Enolase, a ubiquitous enzyme, catalyzes the reversible conversion of 2-phospho­glycerate (2PG) to phospho­enolpyruvate (PEP) in the glycolytic pathway of organisms of all three domains of life. Here we present structural snapshots of Mycobacterium tuberculosis (Mtb) enolase in apo, PEP-bound and two 2PG-bound forms as it catalyzes the conversion of PEP to 2PG. MtEno has a topology similar to other enolase structures, a smaller N-terminal domain and a larger C-terminal domain. The crystal and the cryoEM structures (enzyme in solution, frozen) along with the biochemical studies clearly demonstrate that the functional unit of MtEno is an octamer.

Tautomerization resonance is accelerated on acidification of the carboxyl group of 2PG which is accomplished through its lone-pair-mediated coordination with both the Mg2+ ions and the transfer of a proton from His154 onto the nearest oxygen linked to the phosphate moiety. To find out if the exact reverse of this reaction occurs during the conversion of PEP to 2PG, we systematically mutated each of the residues Ser42, Asp241, Glu163, Glu204 and Lys335 to alanine, compared their activity with wild type MtEno, and elucidated the structures of three of them [Figs. 4(a) and 4(b)]. Notably, the K335A mutation disrupts the nucleophilic (proton) substitution, the E204A mutation defuncts enolation capacity, D241A should make the MgA 2+ coordination in the active site highly improbable and S42A should absolve the MgB 2+ coordination. We analyzed the solvent accessibility in the protein structure based on tunnels and channels buried in the core of the protein by employing CAVER. The water-accessibility channel tunnel of the MtEno S42A–2PG co-crystal structure was similar to that of MtEno Wt-2PG [Figs. 4(d) and 4(e)], corroborating our annotation of the substrate being 2PG. On the other hand, MgB 2+ was absent, possibly owing to the role of Ser42 in MgB 2+ coordination. However, conversion of PEP to 2PG even in its absence indicated that MgB 2+ may be non-obligatory for the reverse reaction. Moreover, the activity of MtEno–S42A is considerably reduced (∼5% of MtEno WT enzyme) but not completely abolished unlike other mutant enzymes which were non-functional [Fig. 4(b)]. Based on these results, it is plausible that, while MgB 2+ aids in the tautomerization, the presence of MgA 2+ makes its presence partially redundant.

> MHHHHHHMPIIEQVRAREILDSRGNPTVEVEVALIDGTFARAAVPSGAATGEHEAVELRDGGDRYGGKGVQKAVQAVLDEIGPAVIGLNADDQRLVDQALVDLDGTPDKSRLGGNAILGVSLAVAKAAADSAELPLFRYVGGPNAHILPVPMMNILNGGAHADTAVDIQEFMVAPIGAPSFVEALRWGAEVYHALKSVLKKEGLSTGLGDEGGFAPDVAGTTAALDLISRAIESAGLRPGADVALALDAAATEFFTDGTGYVFEGTTRTADQMTEFYAGLLGAYPLVSIEDPLSEDDWDGWAALTASIGDRVQIVGDDIFVTNPERLEEGIERGVANALLVKVNQIGTLTETLDAVTLAHHGGYRTMISHRSGETEDTMIADLAVAIGSGQIKTGAPARSERVAKYNQLLRIEEALGDAARYAGDLAFPRFACETK> GSEVAAAQTQYYLKYFNPDIVYPKNARIMLDTGVVVMSMVDGNSTNPNSNMTGWVRVNSASLIFDQSGKTQQEINDSQKQKLPSLKDYGAVSGQDSTAAIKAAIAAEDFLYFGDIGDNFIVSEQIDLRDGCYYVSNGAKFTAALGIEGSQPYTPKSIINASGKVGINISGLVRTHIDHNIFSALGDANSKPTISGFLADAAIDCDFGKWESVGSVNYYYTPNFKEYGIVDLRNSIDCYIEADVNGRWTEETTASTPSTVGIMGSNNKGCYLKGRAKNCYWSGILWEGEDCVVDGPHVRNTKGSNLNLAGKNTAAYNVDLYGSEQGNISIGEGATQAENCNVVGGVAGNAKFANCHLHSVTKNCHVKLFHYGWGQTASAVSDATSGIRCQGTGNTIDSEFDVTYGGLTVKGDAVNVYCSTLTNPEATNIKVNVVGIGARVQIRAPYTIVNAKITGATGDAVVLGERCKGSIVEEVTAIKCGRPLQYAPKTTDANDYAGVIIGRINDVECTNRSVFYGQKIVHSQRKIERIYAQETAFVLDQVLEAIE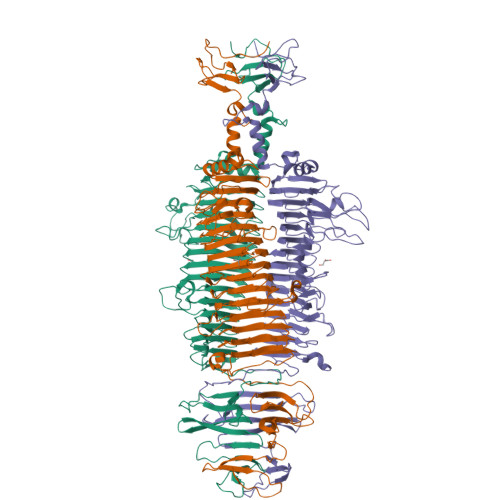VYTNDSGVTGANKLASAIRHISADSFGTSYGLDLVASTISKNNLANSKTKVRAGHIEVEPAVAGAASHIVLYAANGTKWKLEPTGSASAANWVAV> MKNVGFIGWRGMVGSVLMDRMSQENDFENLNPVFFTTSQAGQKAPVFGGKDAGDLKSAFDIEELKKLDIIVTCQGGDYTNEVYPKLKATGWDGYWVDAASALRMKDDAIIVLDPVNQHVISEGLKKGIKTFVGG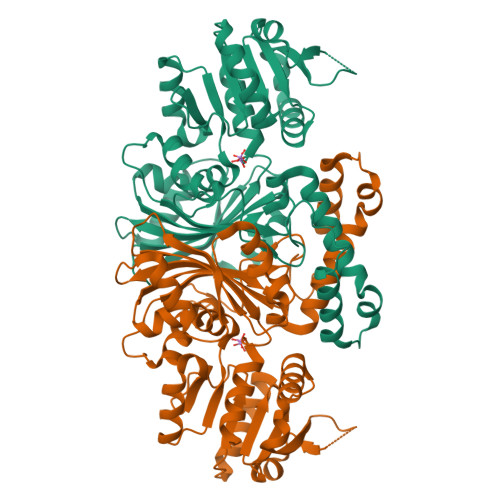NCTVSLMLMAIGGLFEKDLVEWISVATYQAASGAGAKNMRELLSQMGLLEQAVSSELKDPASSILDIERKVTAKMRADNFPTDNFGAALGGSLIPWIDKLLPETGQTKEEWKGYAETNKILGLSDNPIPVDGLCVRIGALRCHSQAFTIKLKKDLPLEEIEQIIASHNEWVKVIPNDKEITLRELTPAKVTGTLSVPVGRLRKLAMGPEYLAAFTVGDQLLWGAAEPVRRILKQLVA>MCTTYTIKSGDTCYAISQARGISLSDFESWNA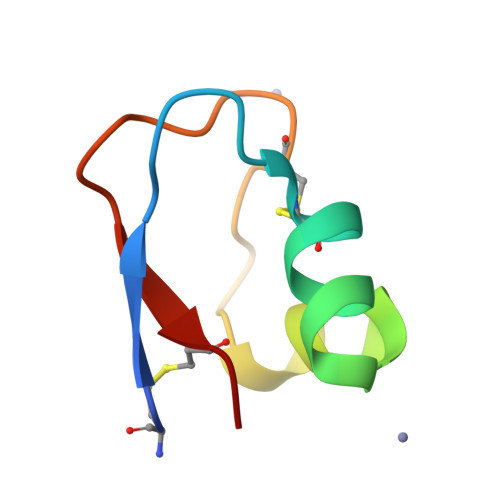GIDCNNLQIGQVVCVSK[4x]>CTRFVYLDPHNPDYPITARSMDWADDTETNLWIFPQELKRSGGAGQYSLEWTSKYGSVIASAFDGRKGMASTTDGVNEKGLAANVLWLAESEYPKTKPTAKKPGLSVAAWAQYVLDNFATVDEAVKSLQQEKFILVTKQVEGQKRLATLHLSLSDSSGDSAIIEYIDGKQVIHHSKNYQVMTNSPTFDQQLTLNAYWDQIGGNVMLPGTNRAADRFVRASFYVKNV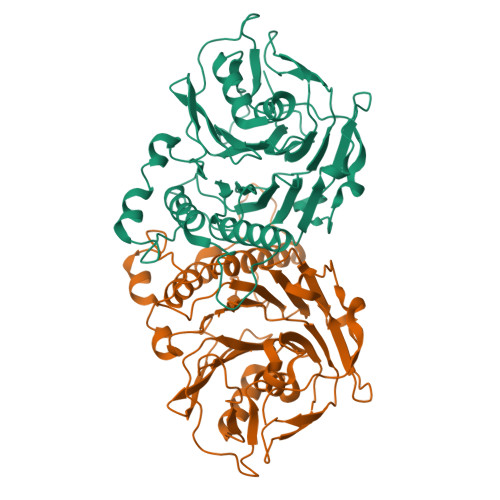NPNKLIPGVAEKGKIEKDKADLATAFSIIRNASVPYGYSLPDMPNIASTRWRTVVDHKSLQYFFESAVSPNIFWVDLKKINFAPRGGSAAKLDLGPNQSTIYSGQASGHFKPAQPFEFAGLLEHHHHHH[8x]>GSHMSPNTVRHRSLVTAQDRPPRGKTVWFTGLSGSGKSSVAMLVERKLLEKGISAYVLDGDNLRHGL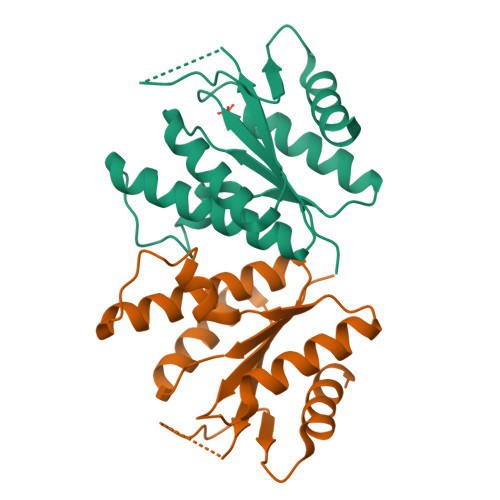NADLGFSMADRAENLRRLSHVATLLADCGHLVLVPAISPLAEHRALARKVHADAGIDFFEVFCDTPLQDSERRDPKGLYAKARAGEITHFTGIDSPYQRPKNPDLRLTPDRSIDEQAQEVIDLLES[2x]>GSRATVFKLGLFKSLFLCSFHDITRLFKNDKTTNQQWVLAVFGLAEVFFEASFELLKKQCSFLQMQKRSHEGGTCAVYLICFNTAKSRETVRNLMANMLNVREECLMLQPPKIRGLSAALFWFKSSLSPATLKHGALPE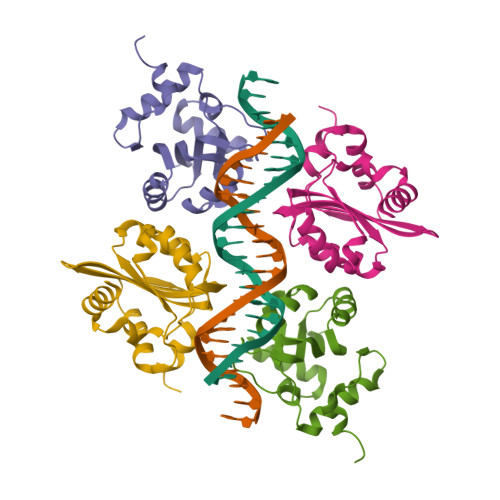WIRAQTTLN[8x]N-[(1S)-1-(AMINOCARBONYL)-4-(ETHANIMIDOYLAMINO)BUTYL]BENZAMIDE 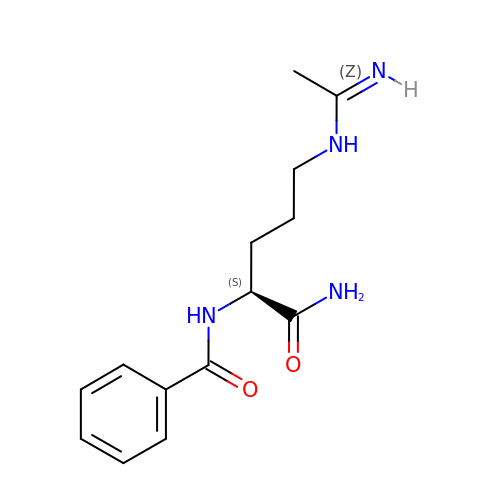| C14 H20 N4 O2 | LWFFSSMDFWZNNW-LBPRGKRZSA-N> AEVLHLCRSLEVGTVMTLFYSKKSQRPERKTFQVKLETRQITWSRGADKIEGSIDIREIKEIRPGKTSRDFDRYQEDPAFRPDQSHCFVILYGMEFRLKTLSLQATSEDEVNMWIKGLTWLMEDTLQAATPLQIERWLRKQFYSVDRNREDRISAKDLKNMLSQVNYRVPNMRFLRERLTDLEQRSGDITYGQFAQLYRSLMYSAQKTMDLPFLETNTLRTGERPELCQVSLSEFQQFLLEYQGELWAVDRLQVQEFMLSFLRDPLREIEEPYFFLDELVTFLFSKENSVWNSQLDAVCPETMNNPLSHYWISSSANTYLTGDQFSSESSLEAYARCLRMGCRCIELDCWDGPDGMPVIYHGHTLTTKIKFSDVLHTIKEHAFVASEYPVILSIEDHCSIAQQRNMAQHFRKVLGDTLLTKPVDIAADGLPSPNQLKRKILIKHKKLAEGSAYEEVPTSVMYSENDISNSIKNGILYLEDPVNHEWYPHYFVLTSSKIYYSEETSSDQGNEDEEEPKEASGSTELHSSEKWFHGKLGAGRDGRHIAERLLTEYCIETGAPDGSFLVRESETFVGDYTLSFWRNGKVQHCRIHSRQDAGTPKFFLTDNLVFDSLYDLITHYQQVPLRCNEFEMRLSEPVPQTNAHESKEWYHASLTRAQAEHMLMRVPRDGAFLVRKRNEPNSYAISFRAEGKIKHCRVQQEGQTVMLGNSEFDSLVDLISYYEKHPLYRKMKLRYPINEEALEKIGTAEPDYGALYEGRNPGFYVEANPMPTFKCAVKALFDYKAQREDELTFTKSAIIQNVEKQDGGWWRGDYGGKKQLWFPSNYVEEMINPAILEPEREHLDENSPLGDLLRGVLDVPACQIAIRPEGKNNRLFVFSISMPSVAQWSLDVAADSQEELQDWVKKIREVAQTADARLTEGKMMERRKKIALELSELVVYCRPVPFDEEKIGTERACYRDMSSFPETKAEKYVNKAKGKK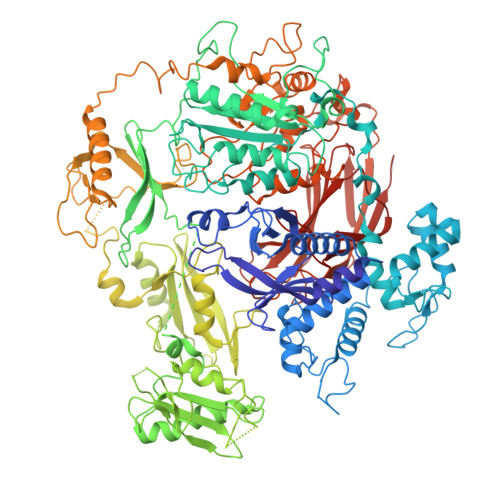FLQYNRLQLSRIYPKGQRLDSSNYDPLPMWICGSQLVALNFQTPDKPMQMNQALFMAGGHCGYVLQPSTMRDEAFDPFDKSSLRGLEPCVICIEVLGARHLPKNGRGIVCPFVEIEVAGAEYDSTKQKTEFVVDNGLNPVWPAKPFHFQISNPEFAFLRFVVYEEDMFSDQNFLAQATFPVKGLKTGYRAVPLKNNYSEDLELASLLIKIDIFPAK>[5x]MRGSHHHHHHGSWETEERPRTREEECHFYAGGQVYPGEASRVSVADHSL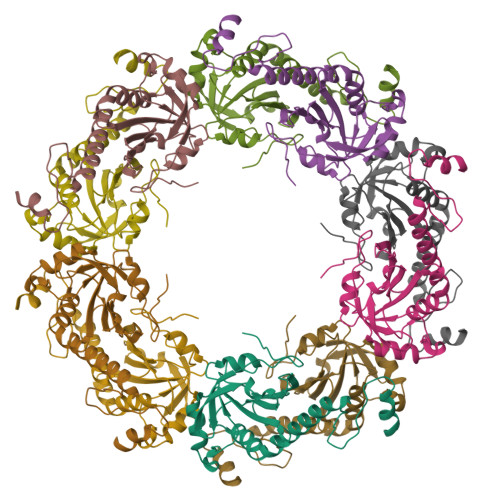HLSKAKISKPAPYWEGTAVIDGEFKELKLTDYRGKYLVFFFYPLDFTFVCPTEIIAFGDRLEEFRSINTEVVACSVDSQFTHLAWINTPRRQGGLGPIRIPLLSDLTHQISKDYGVYLEDSGHTLRGLFIIDDKGILRQITLNDLPVGRSVDETLRLVQAFQYTDKHGEVCPAGWKPGSETIIPDPAGKLKYFDKLN>[2x]AAVIEKRATCSNGKTVGDASCCAWFDVLDDIQQNLFHGGQCGAEAHESIRLVFHDSIAISPAMEAQGKFGGGGADGSIMIFDDIETAFHPNIGLDEIVKLQKPFVQKHG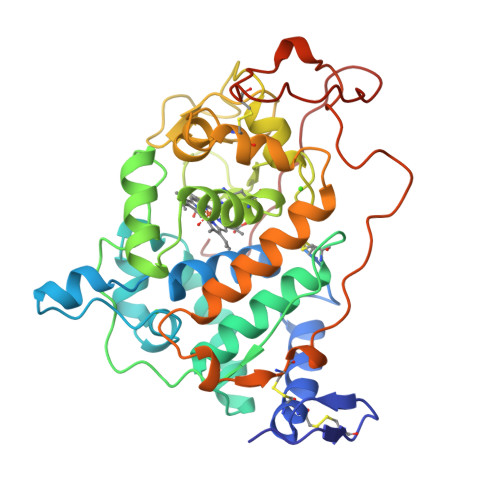VTPGDFIAFAGAVALSNCPGAPQMNFFTGRAPATQPAPDGLVPEPFHTVDQIINRVNDAGEFDELELVFMLSAHSVAAVNDVDPTVQGLPFDSTPGIFDSQFFVETQLRGTAFPGSGGNQGEVESPLPGEIRIQSDHTIARDSRTACEWQSFVNNQSKLVDDFQFIFLALTQLGQDPNAMTDCSDVIPQSKPIPGNLPFSFFPAGKTIKDVEQACAETPFPTLTTLPGPETSVQRIPPPPGA>[2x]MVMMKLFYKPGACSLSPHIVLREAGLDFSIERVDLVTKKTETGADYLSINPKGQVPALVLDDGSLLTEGVAIVQYLADKVPDRHLIAPSGTLSRYHAIEWLNFIATELHKGFSPLFNPNTP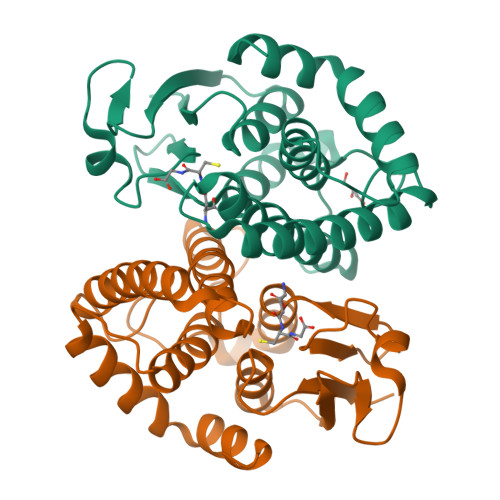DEYKTIVRERLDKQFSYVDSVLAEHDYLLGKKFSVADAYLFTVSRWANALNLQIKERSHLDQYMARVAERPAVKAALAAEDIKAENLYFQ> MGDSKVKVAVRVRPMNRREIDLHTKCVVDVEANKVILNPINTNLSKGDA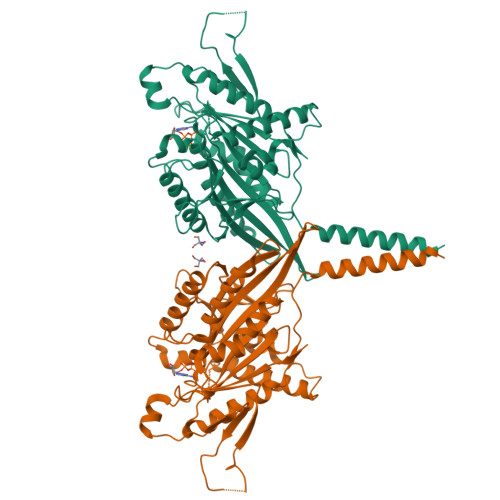RGQPKIFAYDHCFWSMDESVREKYAGQDDVFKCLGENILQNAFDGYNACIFAYGQTGSGKSYTMMGTADQPGLIPRLCSGLFERTQKEENEEQSFKVEVSYMEIYNEKVRDLLDPKGSRQTLKVREHSVLGPYVDGLSKLAVYSYKDIESLMSEGNKSRTVAATNMNEESSRSHAVFKITLTHTLYDVKSGTSGEKVGKLSLVDLAGSERATKTGAAGDRLKEGSNINKSLTTLGLVISALADQGAGKNKNKFVPYRDSVLTWLLKDSLGGNSKTAMVATVSPAADNYDETLSTLRYADRAKHIINHAVVNEDPNARIIRDLREEVEKLREQLTKAEAMKSPELKDRLEESEKLIQEMTVTWEEKLRKTEEIAQERQKQLESHHHHHH>[2x]MVNSSKSILIHAQNKNGTHEEEQYLFAVNNTKAEYPRDKTIHQLFEEQ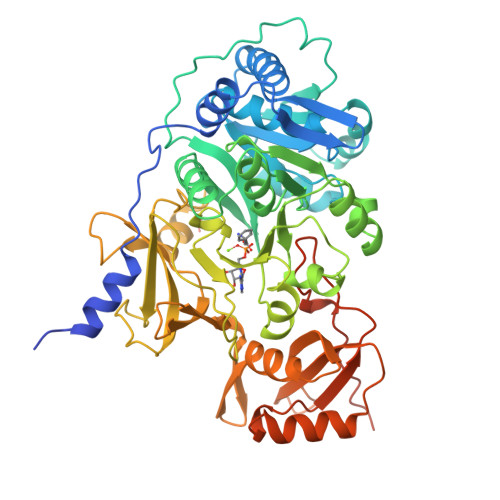VSKRPNNVAIVCENEQLTYHELNVKANQLARIFIEKGIGKDTLVGIMMEKSIDLFIGILAVLKAGGAYVPIDIEYPKERIQYILDDSQARMLLTQKHLVHLIHNIQFNGQVEIFEEDTIKIREGTNLHVPSKSTDLAYVIYTSGTTGNPKGTMLEHKGISNLKVFFENSLNVTEKDRIGQFASISFDASVWEMFMALLTGASLYIILKDTINDFVKFEQYINQKEITVITLPPTYVVHLDPERILSIQTLITAGSATSPSLVNKWKEKVTYINAYGPTETTICATTWVATKETIGHSVPIGAPIQNTQIYIVDENLQLKSVGEAGELCIGGEGLARGYWKRPELTSQKFVDNPFVPGEKLYKTGDQARWLSDGNIEYLGRIDNQVKIRGHRVELEEVESILLKHMYISETAVSVHKDHQEQPYLCAYFVSEKHIPLEQLRQFSSEELPTYMIPSYFIQLDKMPLTSNGKIDRKQLPEPDLTFGMRVDYEAPRNEIEETLVTIWQDVLGSHHHHHH>[2x]MAAPDLLDPKSATHNTKPRLSFSSKPIVYNSGDDCESITTVMKWKTVLAIFLLVVLYLIIGATVFKALEQPEEGLQKYRIIQEKIDFLSMHTCVQTSELEDLVKQVVLAIRAGVNPSGHPSQESSMWDLSSSFFFAGTVITTIGFGNVSPHTEGGRIFCIIYALLGIPLFGFLLAGVGDQLGTIFGKGIAKVEKMFVKWNVSQTKIRVTSTVLFILFGCLLFVALPALIFQHIEGWSALESIYFVVITLTTIGFGDFVAGGSEIEYLDYYKPIVWFWILVGLAYFAAVLSMIGDWLRVISKKTKEEVGEFRAHAAEWTANV

Tandem pore domain (K2P) potassium channels modulate resting membrane potentials and shape cellular excitability. For the mechanosensitive subfamily of K2Ps (including the TREK1, TREK2, and TRAAK channels), diverse stimuli control channel activity, including lipids, pH, heat, membrane tension, post-translational modification, and an array of pharmacologically active agents including volatile anesthetics, antidepressants, and neuroprotective agents. Two key regions of the mechanosensitive K2P channel structure appear to control channel function, the conformationally flexible TM4 helix, and the selectivity filter. Overall, this cryo-EM structure exhibits K2P architectural features consistent with prior crystallographic studies: a dimeric channel assembly with each subunit composed of four transmembrane helices, a domain-swapped cap located above the selectivity filter, and an extended membrane facing TM2/TM3 loop within each subunit.

Using single particle cryo-EM, we first solved a 3.27 Å resolution structure of TREK1 solubilized in DDM detergent in an unexpected conformation. However, unlike all prior TREK1 structures, where intermolecular crystallization contacts immobilize the TM4 helix in an “up” conformation, the TM4s in our cryo-EM samples are unconstrained prior to sample vitrification. As a result, we find that TREK1 exhibits a previously unobserved asymmetric TM4 “up/down” conformational state. This asymmetry is due to an ~11° bend in the TM4a helix in the “up” state relative to the TM4b helix in the “down” state. The apparent cause of the observed TREK1 TM4 asymmetry is the presence of a density non-contiguous with the TREK1 density map but near the TM4b helix, sterically impeding TM4b from adopting the “up” conformation (pink). This density extends directly below the TREK1 selectivity filter, occluding the ion permeation pathway. The TREK1 protein is solubilized in n-dodecyl-β-d-maltoside (DDM) detergent and a molecule of DDM easily fits the observed density if the DDM is oriented with its maltoside sugar moieties located within the pore and hydrocarbon tail projecting outward toward the fenestration. While the positioning of this pore-bound DDM molecule is inverted relative to the orientation of DDM molecules in the micelle surrounding the TREK1 protein, the presence of a detergent molecule within the TREK1 pore suggested that this site could be a target for lipids in a biological membrane. Native MS analyses of DDM-purified TREK1 showed intact TREK1 dimer with a charge distribution similar to results previously observed for TRAAK in DM detergent, but did not identify any lipids bound to the TREK1 protein. While prior structures of TRAAK channels also exhibited asymmetric positioning of the TM4 helices, this asymmetry has always been attributed to crystallization artifacts and has not been considered biologically relevant.>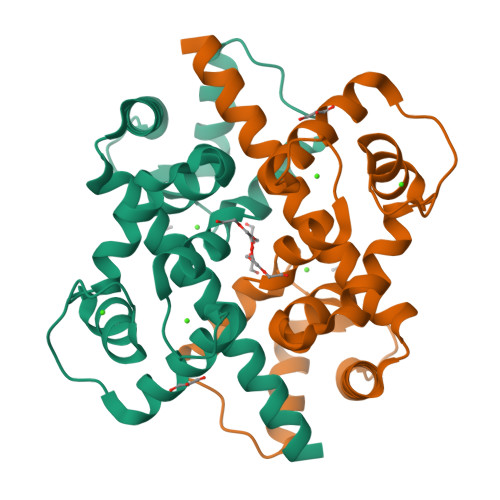 MHHHHHHSSGRENLYFQGIHVLENFKNYGLLLKFQKLAMTIIAQQSNDYDVEKLKSTFLVLDEDGKGYITKEQLKKGLEKDGLKLPYNFDLLLDQIDSDGSGKIDYTEFIAAALDRKQLSKKLIYCAFRVFDVDNDGEITTAELAHILYNGNKKGNITQRDVNRVKRMIRDVDKNNDGKIDFHEFSEMMKL> MNKPIKNIVIVGGGTAGWMAASYLVRALQQQANITLIESAAIPRIGVGEATIPSLQKVFFDFLGIPEREWMP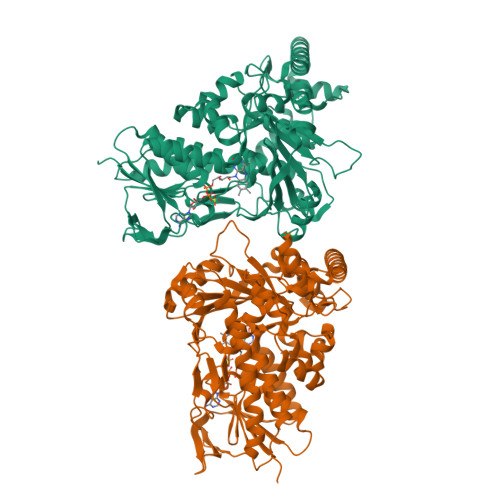QVNGAFKAAIKFVNWRKSPDPSRDDHFYHLFGNVPNCDGVPLTHYWLRKREQGFQQPMEYACYPQPGALDGKLAPCLSDGTRQMSHAWHFDAHLVADFLKRWAVERGVNRVVDEVVDVRLNNRGYISNLLTKEGRTLEADLFIDCSGMRGLLINQALKEPFIDMSDYLLCDSAVASAVPNDDARDGVEPYTSSIAMNSGWTWKIPMLGRFGSGYVFSSHFTSRDQATADFLKLWGLSDNQPLNQIKFRVGRNKRAWVNNCVSIGLSSCFLEPLESTGIYFIYAALYQLVKHFPDTSFDPRLSDAFNAEIVHMFDDCRDFVQAHYFTTSRDDTPFWLANRHDLRLSDAIKEKVQRYKAGLPLTTTSFDDSTYYETFDYEFKNFWLNGNYYCIFAGLGMLPDRSLPLLQHRPESIEKAEAMFASIRREAERLRTSLPTNYDYLRSLRDGDAGLSRGQRGPKLAAQESL> YPKPD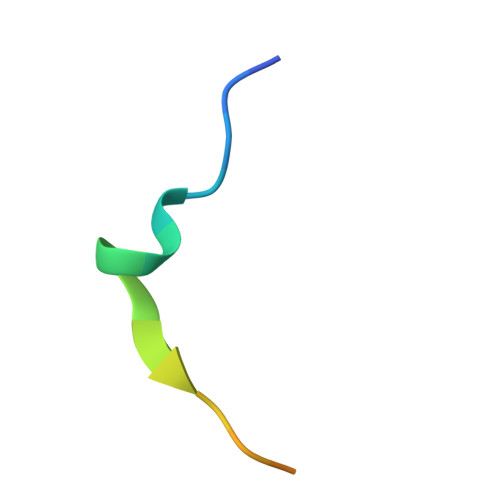TQQMIPFQPRHLAPP>[2x]MELIQDTSRQPLEYVKGVPLIKYFAEALGPLQSFQARPDDLLISTYPKSGTTWVSQILDMIYQGGDLEKCHRAPIFNRVPFLEFKAPGIPSGMETLKDTPAPRLLKTHLPLALLPQTLLDQKVKVVYVARNAKDVAVSYYHFYHMAKVHPDPGTWDS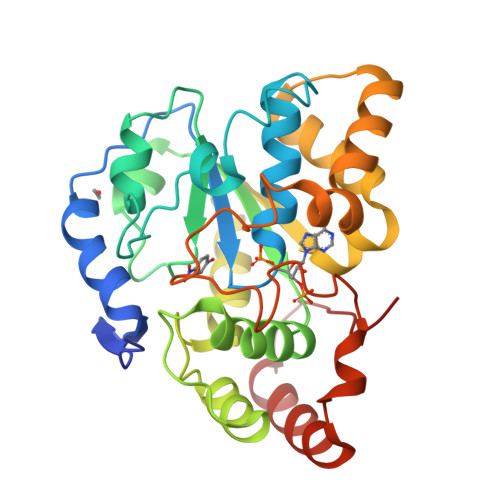FLEKFMVGEVCYGSWYQHVQEWWELSRTHPVLYLFYEDMKENPKREIQKILEFVGHSLPEETVDFMVQHTSFKEMKKNPMTNYTTIPQEIMDHSISPFMRKGMAGDWKTTFTVAQNERFDADYAEKMAGCSLSFRSEL> MSEVINFDQIFEGAIEPGKEPKRLFKEVYEGAITATSYAEILLSRAIEKYGPDHPVGYPDTAYFLPVIRAFSGEEVRTLKDMVPILNRMRAQIKSELTFENARLAGEATWYAAEIIEALRYLKHTPENPIVVP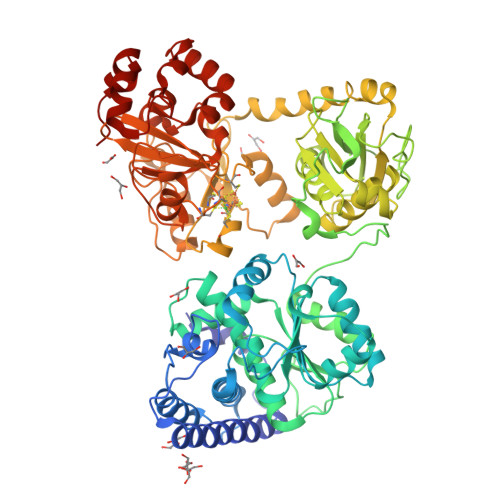PWTGFIGDPVVRQYGIKMVDWTIPGEAIIIGRAKDSKAAKKIVDDLMGKGLMLFLCDEIIEQLLEENVKLGVDYIAYPLGNFTQVVHAANYALRAGLMFGGIAPGLRDAHRDYQRRRVLAFVLYLGEHDMVKTAAAMGAIFTGFPVITDQPLPEDKQIKDWFISEPDYDKIVQTALEVRGIKITSIDIDLPINFGPAFEGESIRKGDMHVEFGGGKTPSFELVRMVGPDEIEDGKVEVIGPDIDSVEPGGRLPIGIVVDIYGRKMQEDFEPVLERRIHYFTNYGEGFWHTAQRDLTWVRISKEAFAKGARLKHLGQLLYAKFKQEFPSIVDRVQVTIYTDEQKVLELREIARKKYAERDARLRELSDEAVDTYYSCLLCQSFAPTHVCIVSPERVGLCGAISWLDAKAAYEINPNGPNQPIPKEGLIDPVKGQWESFNEYIYKNSQRTIERMNLYTIMEYPMTSCGCFEAIMAYLPELNGFMIVNREHSGMTPIGMTFSTLAGMVGGGTQTPGFMGIGKSYIGSRKFVKADGGLARVVWMPKDLKEQLRSIIEERAEEEGLGRDFIDKIADETVGTTVDEVLPFLEEKGHPALSMEPLL>MGSSHHHHHHSSENLYFQGHMNEIYQKAKHIKLFAMDVDGILSDGQIIYNSEGTETKA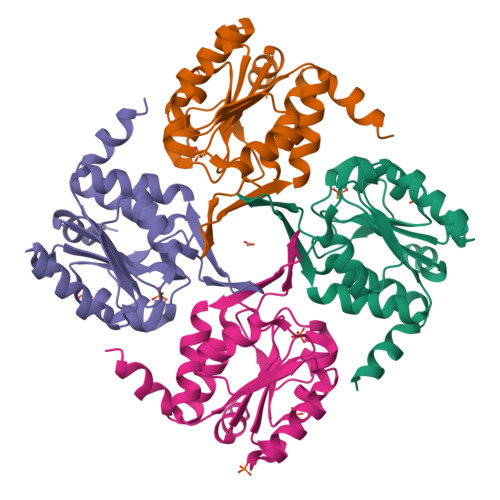FYVQDGLGLQALKQSGIILAIITGRSSAMVDRRAKELGISHIIQGQDDKLTALVGLTKKLGIELSHCAYIGDDLPDLKAVREAGFGISVPNGCEQTRAVSDYITTKTGGNGAVREVCELILKAQNNFDAFIATFQ[4x]~{N}-(2,3-dimethylphenyl)-5-(4-pyridin-4-yloxyphenyl)-4~{H}-1,2,4-triazol-3-amine 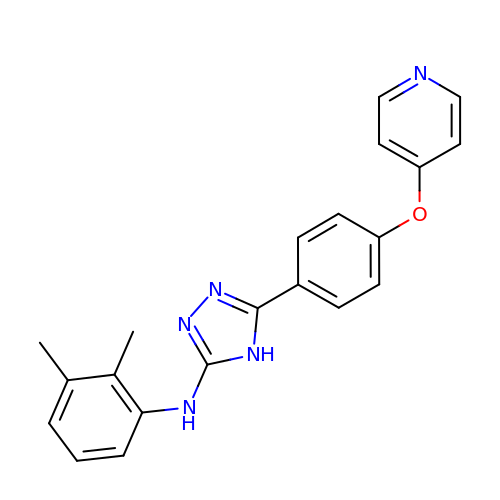| C21 H19 N5 O | FRUZWHLTFSTCFH-UHFFFAOYSA-N>MFFNKKNNQDELKKLAATEAAKSITTEITLGVGTGSTVGFLIEELVNYRDKIKTVVSSSEDSTRKLKALGFDVVDLNYAGEIDLYIDGADECNNHKELIKGGGAALTREKICVAAAKKFICIIDESKKVNTLGNFPLPIEVIPMARSYIARQIVKLGGQPVYR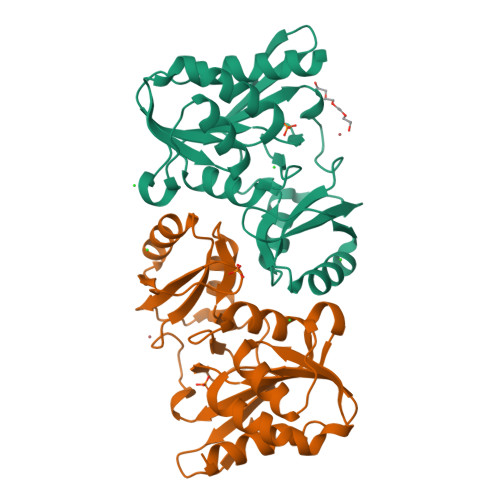EQTITDNGNVILDVYNLKIDNPLKLETELNQITGVVTNGIFALKPADTVIMATKDSNIVVL[2x]>[2x]TDLIQRPRRLRKSPALRAMFEETTLSLNDLVL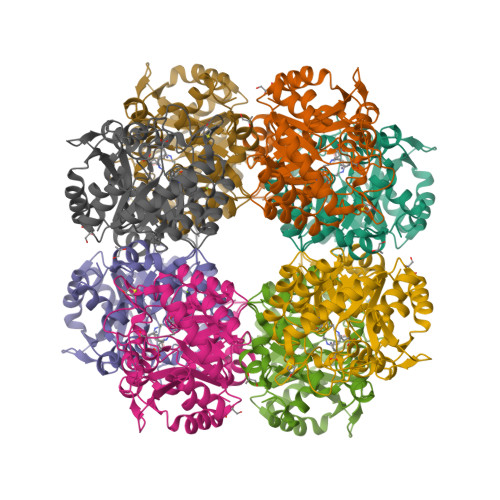PIFVEEEIDDYKAVEAMPGVMRIPEKHLAREIERIANAGIRSVMTFGISHHTDETGSDAWREDGLVARMSRICKQTVPEMIVMSDTCFCEYTSHGHCGVLCEHGVDNDATLENLGKQAVVAAAAGADFIAPSAAMDGQVQAIRQALDAAGFKDTAIMSYSTKFASSFYGPFREAAGSALKGDRKSYQMNPMNRREAIRESLLDEAQGADCLMVKPAGAYLDIVRELRERTELPIGAYQVSGEYAMIKFAALAGAIDEEKVVLESLGSIKRAGADLIFSYFALDLAEKKILR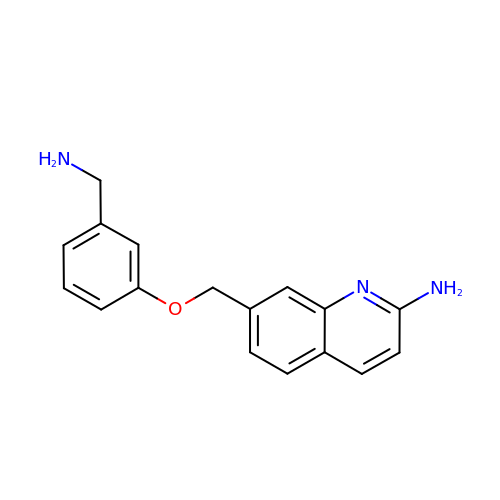7-[[3-(aminomethyl)phenoxy]methyl]quinolin-2-amine | C17 H17 N3 O | ADYDYORVGGQJTJ-UHFFFAOYSA-N> MFISRHSGEGKFLFIDQRATLVIGFLPQEILGTSFYEYFHNEDIAALMESHKMVMQVP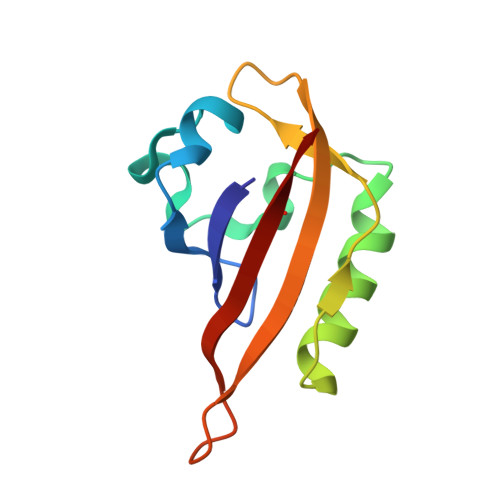EKVTTQVYRFRCKDNSYIQLQSEWRAFKNPWTSEIDYIIAKNSVF> GHMTWKPNVTVAAVIEQDDKYLLVEEIPRGTAIKLNQPAGHLEPGESIIQACSREVLEETGHSFLP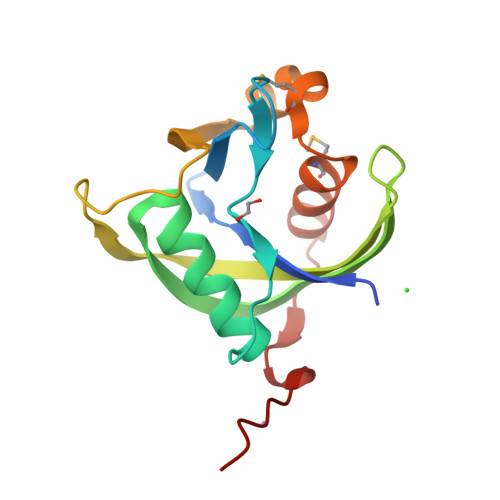EVLTGIYHWTCASNGTTYLRFTFSGQVVSFDPDRKLDTGIVRAAWFSIDEIRAKQAMHRTPLVMQCIEDYHAGKRYPLDILQYYDGS> DFTVSTTEDLQRFRNECVSSLSVPADYVEKFKKWEFPEDDTTMCYIKCVFNKMQLFDDTEGPLVDNLVLQLAHGRDGEEVRTEV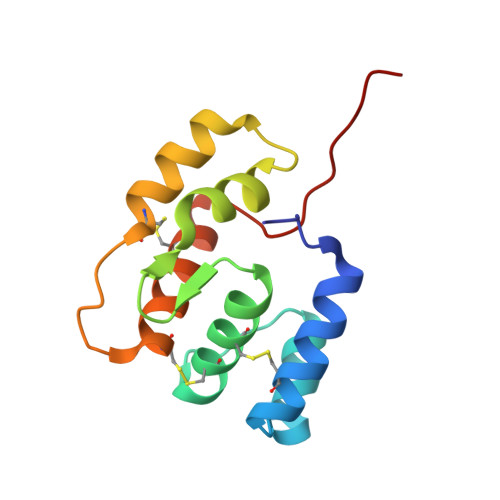MKCVDKNTDNNACHWAFRGFKCFQKNNLSLIKASIKKD> GEIRPTIGQQMETGDQRFGDLVFRQLAPNVWQHTSYLDMPGFGAVASNGLIVRDGGRVLVVDTAWTDDQTAQILNWIKQEINLPVALAVVTHAHGDKMGGMDALHAAGIATYANALSNQLAPQEGMVAAQHSLTFAANGWVEPATAPNFGPLKVFYPGPGHTSDNITVGIDGTDIAFGGCLIKDSKAKSLGNLGDADTEHYAASARAFGAAFPKASMIVMSHS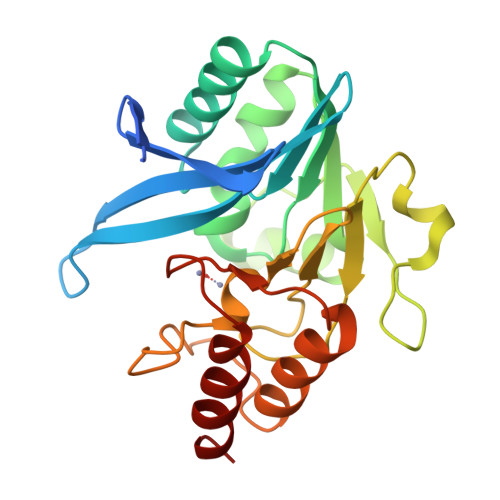APDSRAAITHTARMADKLR>AASSLDELVALCKRRGFIFQSSEIYGGLQGVYDYGPLGVELKNNLKQAWWRRNVYERDDMEGLDASVLTHRLVLHYSGHEATFADPMVDNAKARYWTPPRYFNMMFQDLRGPRGGRGLLAYLRPETAQGIFVNFKNVLDATSRKLGFGIAQIGKAFRNEITPRNFIFRVREFEQMEIEYFVRPGEDEYWHRYWVEERLKWWQEMGLSRENLVPYQQPPESSAHYAKATVDILYRFPHGSLELEGIAQRTDFDLGSHTKDQEALGITARVLRNEHSTQRLAYRDPETGKWFVPYVIEPSAGVDRGVLALLAEAFTREELPNGEERIVLKLKPQLAPIKVAVIPLVKNRPEITEYAKRLKARLLALGLGRVLYEDTGNIGKAYRRHDEVGTPFAVTVDYDTIGQSKDGTTRLKDTVTVRDRDTMEQ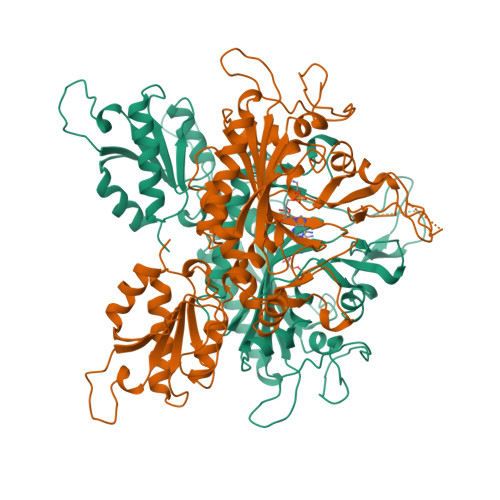IRLHVDELEGFLRERLRW[2x]A related group of proteins with a similar Mn/Fe cofactor is termed R2-like ligand-binding oxidases (R2lox). Following O2 activation, their cofactor catalyzes a two-electron redox reaction which results in the formation of a tyrosine–valine ether cross-link in the protein. The tyrosine and valine residues are conserved in the R2lox group, and the cross-link was observed in both R2lox proteins that have been structurally characterized. Both proteins also comprise a hydrophobic channel leading to the metal cofactor wherein a long-chain fatty acid molecule is found, which coordinates at the Mn/Fe ions of the cofactor. The mixed-metal cofactor in R2lox self-assembles with the manganese ion in metal-binding site 1 and the iron ion in site 2 if both MnII and FeII are available.

Moreover, A171, which lines the fatty-acid binding tunnel, was changed to phenylalanine (A171F). The latter mutation was designed to create a cofactor geometry in R2lox more closely resembling the R2c site by blocking access of the fatty acid ligand that co-purifies with the wild-type protein and coordinates both metal ions. In A171F-R2lox, the fatty acid is excluded from the active site because the bulky phenylalanine side chain blocks the ligand-binding tunnel. Electron density for a hydrophobic ligand is observed further up in the tunnel, but it could only reasonably be modeled (as caprylic (C8) acid) in the oxidized state. In contrast, in the oxidized state of A171F-R2lox, E167 is a monodentate ligand to Fe2 as in the wild-type, whereas E202 adopts the oxidized or reduced state conformation in roughly equal proportions. However, cofactor oxidation by O2 appears to have taken place regardless of the E202 conformation, because an oxo/hydroxo bridge is clearly observed in the electron density in the position occupied by the fatty acid head group in the wild-type. It appears likely that in those molecules in which E202 is in the oxidized state conformation, a second oxo/hydroxo species occupies the bridging position. Accordingly, the A171F-R2lox cofactor can adopt a geometry which is similar to the oxidized cofactor in R2c, with two oxygen bridges instead of only one as in wt-R2lox. However, none of these structural changes seem to have an effect on cofactor reactivity with respect to cross-link formation. Judging from the electron density, the cross-link was formed equally efficiently in the presence of O2 in A171F-R2lox as in the wild-type protein (inset).

> MAHHHHHHVDDDDKMVHHDGFQTVKATIDWEHPMFKLYEKAKRNGKWNPADIDFSQDQKDFASLTSEEKISALPLVAGFSAGEEAVTLDILPMAHALARQGRLEDVLFLTTFMHDEAKHVEMFSRWQQAVGIGQMDLSVFHNDHYKRIFYEALPEAMNRLYADDSPEAVIRAATVYNMIVEGTLFESGYYTFRQIYKKAGLFPGLLQGIDYLNMDEGRHIQFGIYTIQRIVNEDERYYELFIRYMDELWPHVIGYVDYLTELGKRQQQLARTYALEIDYDLLRHYVIKQFNLRKKQISRTKRVDVVEGLEKTAAES> RSSRTRRE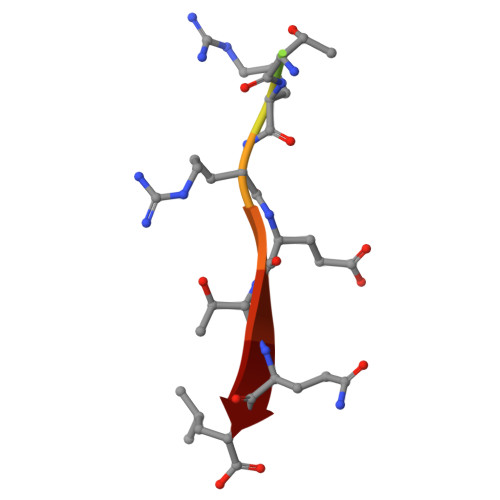TQL>[3x]MAQFFIHRPIFAWVIALVIMLAGILTLTKMPIAQYPTIAPPTVTIAATYPGASAETVENTVTQIIEQQMNGLDGLRYISSNSAGNGQASIQLNFEQGVDPDIAQVQVQNKLQSATALLPEDVQRQGVTVTKSGASFLQVIAFYSPDNNLSDSDIKDYVNSSIKEPLSRVAGVGEVQVFGGSYAMRIWLDPAKLTSYQLTPSDIATALQAQNSQVAVGQLGGAPAVQGQVLNATVNAQSLLQTPEQFKNIFLKNTASGAEVRLKDVARVELGSDNYQFDSKFNGKPAAGLAIKIATGANALDTAEAVEQRLSELRKNYPTGLADKLAYDTTPFIRLSIESVVHTLIEAVILVFIVMFLFLQNWRATIIPTLAVPVVVLGTFAVINIFGFSINTLTMFAMVLAIGLLVDDAIVVVENVERVMSEDHTDPVTATSRSMQQISGALVGITSVLTAVFVPMAFFGGTTGVIYRQFSITLVTAMVLSLIVALTFTPALCATILKQHDPNKEPSNNIFARFFRSFNNGFDRMSHSYQNGVSRMLKGKIFSGVLYAVVVALLVFLFQKLPSSFLPEEDQ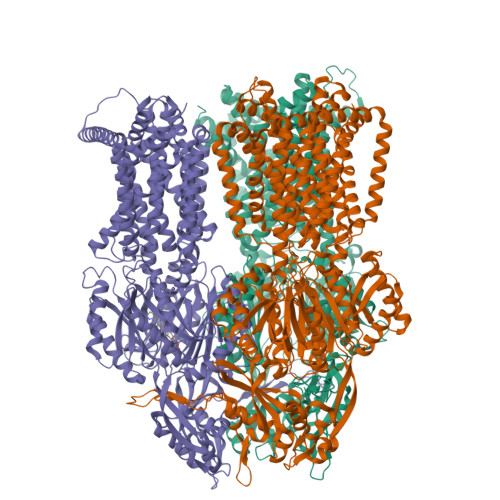GVVMTLVQLPPNATLDRTGKVIDTMTNFFMNEKDTVESIFTVSGFSFTGVGQNAGIGFVKLKDWSKRTTPETQIGSLIQRGMALNMIIKDASYVMPLQLPAMPELGVTAGFNLQLKDSSGQGHEKLIAARNTILGLASQDKRLVGVRPNGQEDTPQYQINVDQAQAGAMGVSIAEINNTMRIAWGGSYINDFVDRGRVKKVYVQGDAGSRMMPEDLNKWYVRNNKGEMVPFSAFATGEWTYGSPRLERYNGVSSVNIQGTPAPGVSSGDAMKAMEEIIGKLPSMGLQGFDYEWTGLSLEERESGAQAPFLYALSLLIVFLCLAALYESWSIPFSVLLVVPLGVIGAIVLTYLGMIIKGDPNLSNNIYFQVAIIAVIGLSAKNAILIVEFAKELQEKGEDLLDATLHAAKMRLRPIIMTTLAFGFGVLPLALSTGAGAGSQHSVGFGVLGGVLSATFLGIFFIPVFYVWIRSIFKYKPKTINTQEHKS>[6x]MRTRSNITTKNGIHWYYEQEGSGPHVVLIPDGLGECKMFDKPMSLIANSGFTVTTFDMPGMSRSSEAPPETYQEITAQKLASYVISICDELAIDKATFWGCASGGCTVLALVADYPTRVRNALAHEVPTYLMEDLKPLLEMDDEAVSAAMSSNVVVGSVGDIEGSWQELGEEAHARLWKN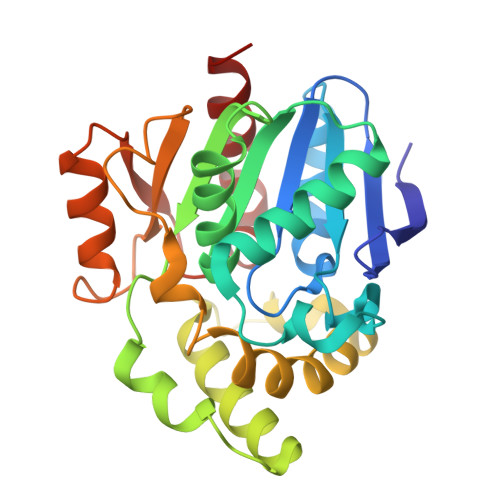YPRWARGYPGYIPQSTPVSKEDLIKAPLDWTVGASTPTARFLDNIVTATKHNIPFQTLPGMHFPYVTHPEVFAEYVVEKTRKYL(1R,3AS,4R,8AS,8BR)-4-(2-BENZO[1,3]DIOXOL-5-YLMETHYL)-1-BENZYL-3-OXO-DECAHYDRO-PYRROLO[3,4-A]PYRROZILIN-4-YL-BENZAMIDINE 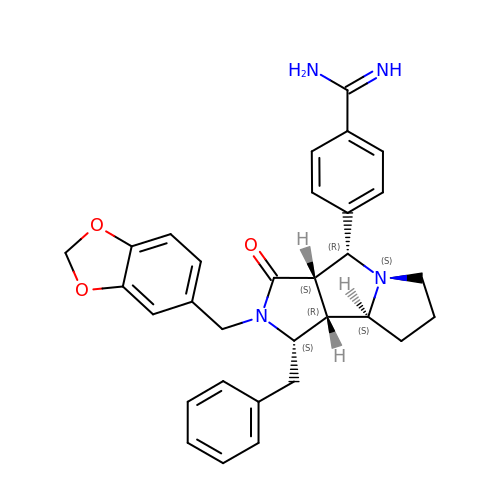| C31 H32 N4 O3 | APELQVQIJUTSME-UDOPOUDQSA-N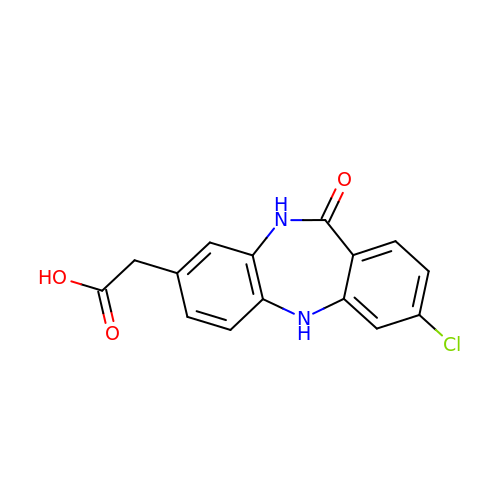(3-chloro-11-oxo-10,11-dihydro-5H-dibenzo[b,e][1,4]diazepin-8-yl)acetic acid | C15 H11 Cl N2 O3 | MFBFXFHWNXYFCJ-UHFFFAOYSA-N>GPHMLEIPKDRRENLQKKLFHMQQLLPNSGLPNLDRWHSLFPLDTKATRNSTCFGYPSWMYKAQNNKNGRHFALRRIEGYRLTNEKAILNVTKEWKKIINANIVTVHEAFTTEFFGDSSLIFVYDFHPLSETLYDHHFPPNNSHNRLRNTNKIPENLLWSYVCQIANALLAIHNAKLAARCLELSKIIWENNRIRLAACSILDVLHHDSPNRKTIEELQQEDFVKFGRIILALATNTPTLNFNNIDAALATIVP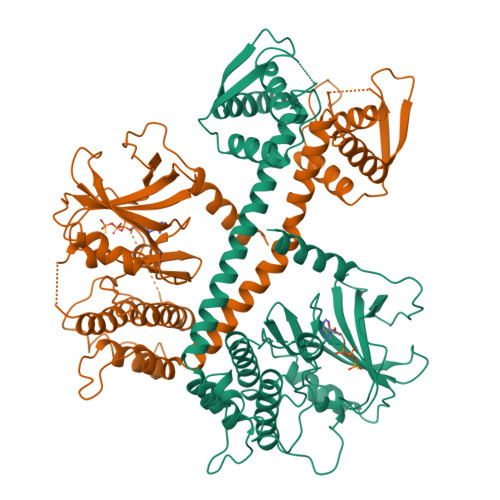RYSTQLRGVLEWLIKPSAPGETKTVETLLGGITTHLANFANFVMQESDEKEFHLMRELENGRIARLMFKLSVVNERGDSCGVHNWSETGERLLLKLFRDYVFHQVDADGKARLDTNHYLNCLSKLDASSEEQILLTSRDNATVFVVSYRSIRQMLDRAYGELGKESKPSATGATI[2x]>CGATC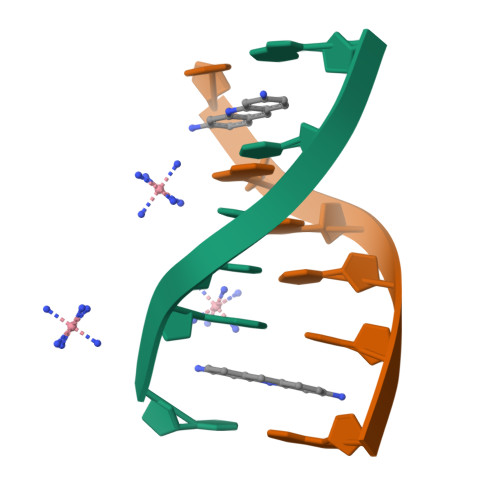G[2x]>[2x]GPGSGMATIEDIKETALIPFQKHRQLSMHEAEVITLEIIGLLCDSECKDEKTLKYLGRFLTPDMYQDLVDERNL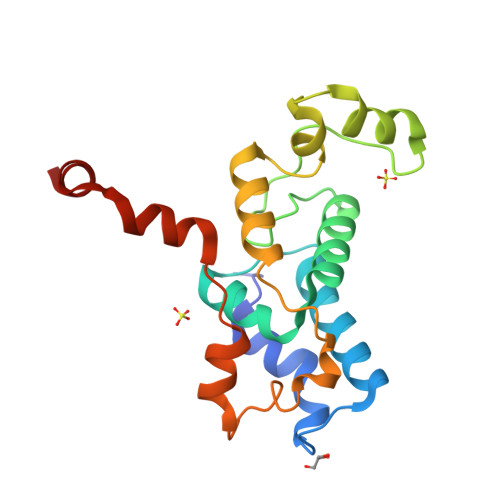NKRCGYPLCGKSPERIRDPFSMNDTTKKFLLENNPYAYLSHYCSKFHFRCSQFYQVQLSDEALFARTGVHLFEDPEQDKHDIDFKVTLFEELLREKASEEDIKSLISGL> GSHMASLDMAEIKEKICDYLFNVS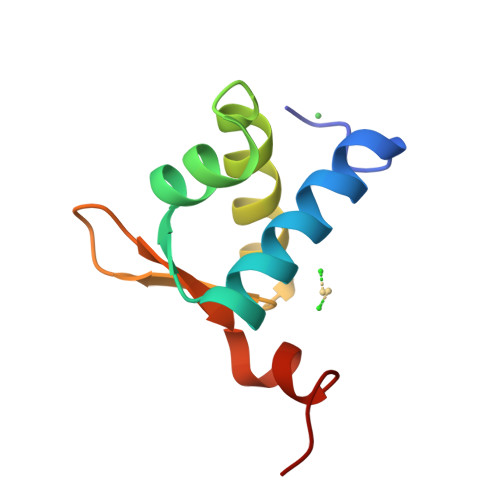DSSALNLAKNIGLTKARDINAVLIDMERQGDVYRQGTTPPIWHLTDKKRERMQIK>[2x]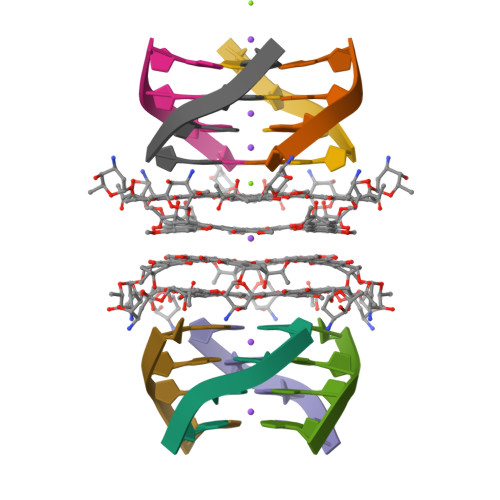GGGG>[2x]MPAEYRYKIVMLGDGAVGKTAMTTRFTQNFFDTDYKRTIGSDFAVKRLQLDDINAHVTLQIWDLAGQPRFESVR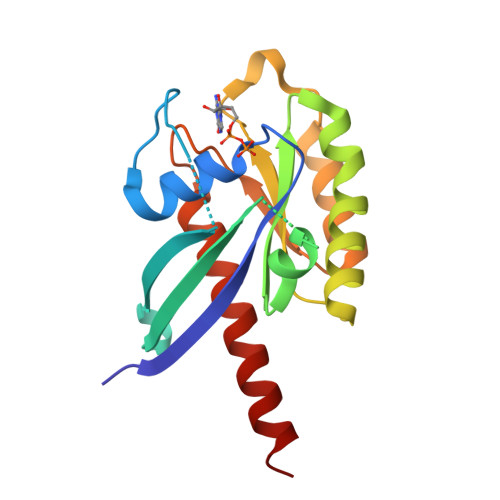QGFYRGARGGLLLYDVTRRRTFINIENWKEEAFRSLQKEIPLVVVANKVDLKDSRVVATEEGEEYAKNNSFMYVESSALTGENVEEAYANLCRIMIEESKDISEMTST9-cyclopentyl-N~8~-(2-fluorophenyl)-N~2~-(4-methoxyphenyl)-9H-purine-2,8-diamine | C23 H23 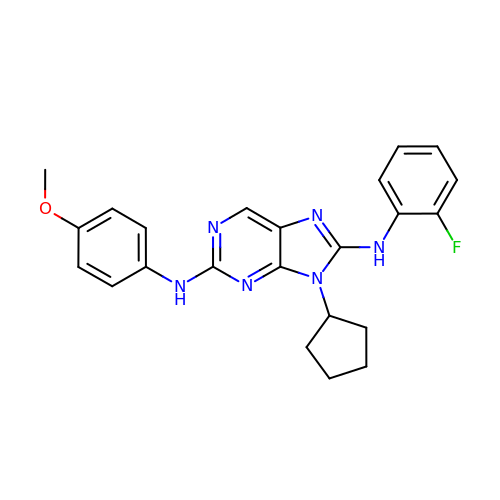F N6 O | IMFVPVKPQOQCBY-UHFFFAOYSA-N> QPQSGPQTGVVFRNTVTGEALDVSQGKEGGRDTPAVKKFLETGENLYIDDKSCLRNGESLFATSCSGCHGHLAEGKLGPGLNDNYWTYPSNTTDVGLFATIFGGANGMMGPHNENLTPDEMLQTIAWIRHLYTGPKQDAV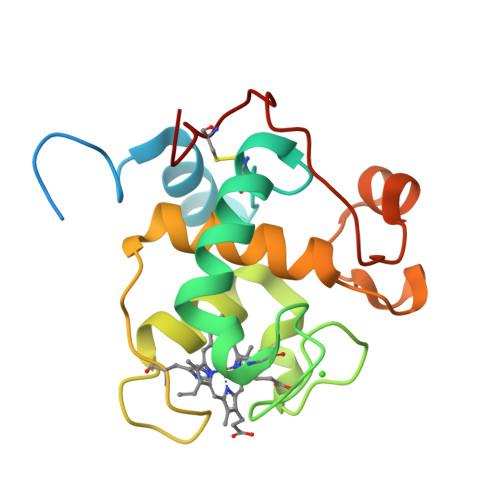WLNDEQKKAYTPYKQGEVIPKDAKGQCKPLDE> TKQ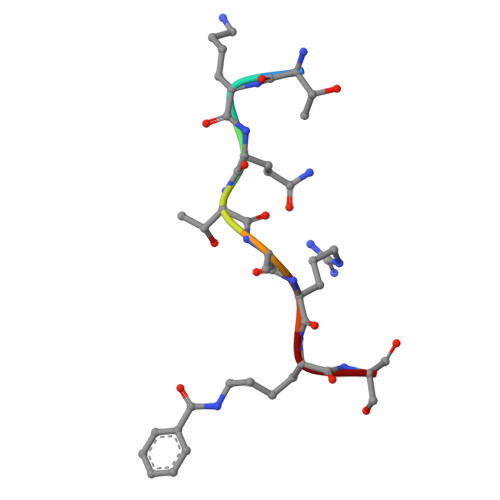TARKS7-(CARBOXYAMINO)-8-AMINO-NONANOIC 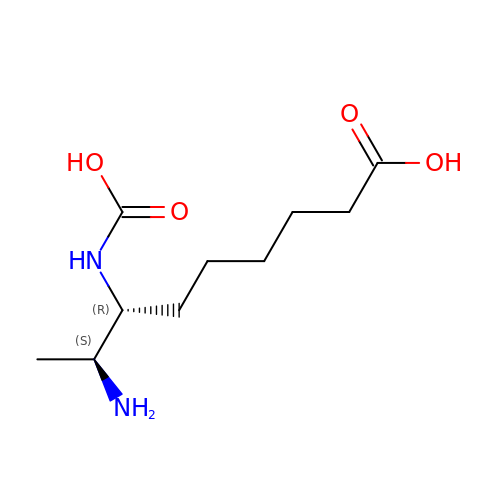ACID | C10 H20 N2 O4 | OQNJZSIPDMTUAJ-JGVFFNPUSA-N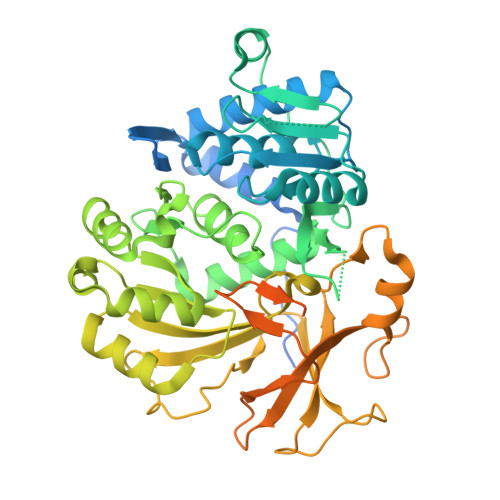> GSHMASMTGGQQMGRGSEFDSERPLCAFDLLGDAERAALAAHNATRHPLAEHTLTALVDAAAHTHADRVALIADGIRLTYREVHDRAGRLAALLAERGVAPGDVVAVALPRSADLVIALLGVLRAGAAYLPLDVDHPPARLAAMVERARAGTVVTCQGALPRLGDRLPGTVVVDDAATRDRLAGLEPLPTRDVHPDQLAYTIFTSGSTGEPKGVGVAHRAIANRLQWMQHTYRLTPEDRVAQKTPVGFDVSVWEFFWPLITGATLVVARPGGHRDPAYLAALFAEHKVTVCHFVPSLLRVFLNEPTARRATALRQVIVSGEALDADLARAWARTLPQARLDNLYGPTEAAVDVTSHPVCGAGTEPVRDPVPIGRPVWNTELYVLDSSLRPLPTGAVGELYLGGVQLARGYVGRPGMTASRFVANPFGPPGSRLYRTGDLVRRRADGAVEYLGRVDDQVKINGVRVEPGEVEAVLRAQPGVADAAVAARPAPAGGLRLVGYLVPDGSPPDVDEVRRGLADRLPAAWVPAAFVVVDALPLTVNGKLRRDALPDPDPGPV>[8x]MSIVNILSVNVLNNPAKFSDPYKFEITFECLEPLKSDLEWKLTYVGSATSQSYDQILDTLLVGPIPIGINKFVFEADPPNIDLLPQLSDVLGVTVILLSCAYEDNEFVR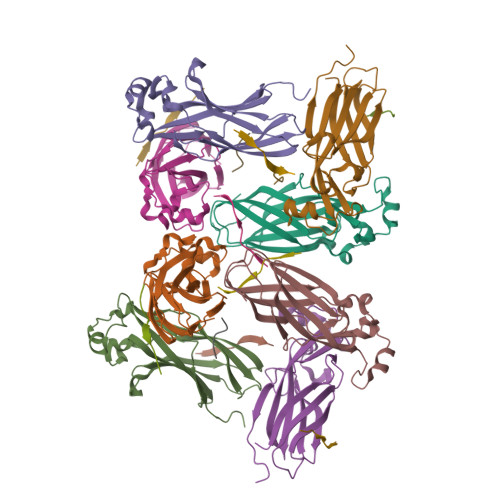VGYYVNNEMEGLNLQEMDDAEIKKVKVDISKVWRSILAEKPRVTRFNIQWDN;>[11x]RKVESSKVSKKRIAPTPVYP>[12x]MKRYVVGISGASGIVLAVTLVSELARLGHHID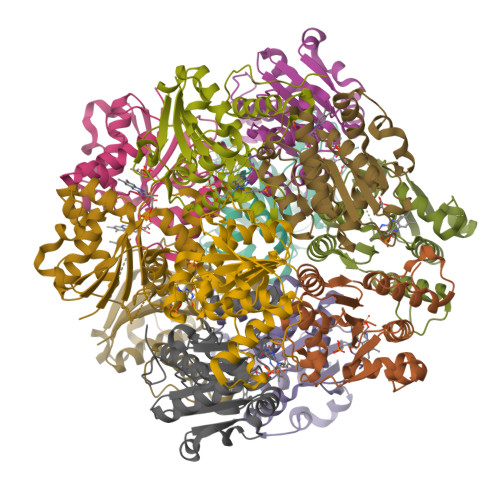VIISPSAQKTLYYELDTKSFLSTIPQNFHNQIVLHHISSIESSVSSGSNTIDATIIVPCSVATVAAISCGLADNLLRRVADVALKEKRPLILVPREAPLSAIHLENLLKLAQNGAVILPPMPIWYFKPQTAEDIANDIVGKILAILQLDSPLIKRWENPRLEHHHHHH> MKRVEDWIKQAERDLEEARYAKSGGYYELACFLSQQCAEKAVKGLLQFQGIEKR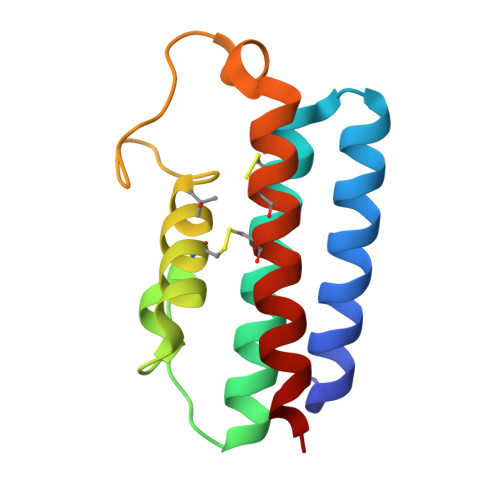GHSISHLLTNPPADILQCATFLDKQYTPSRYPDVYYEGAPYEYYTERDADECINCAIRILNWVKGQIK> MMVAWWSLFLYGLQVAAPALAATPADWRSQSIYFLLTDRFARTDGSTTATCNTADQKYCGG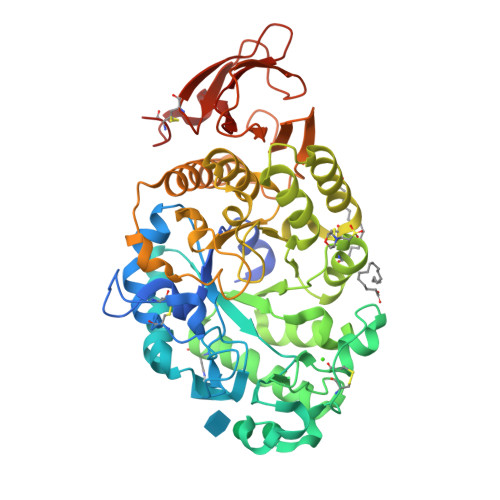TWQGIIDKLDYIQGMGFTAIWITPVTAQLPQTTAYGDAYHGYWQQDIYSLNENYGTADDLKALSSALHERGMYLMVDVVANHMGYDGAGSSVDYSVFKPFSSQDYFHPFCLIQNYEDQTQVEDCWLGDNTVSLPDLDTTKDVVKNEWYDWVGSLVSNYSIDGLRIDTVKHVQKDFWPGYNKAAGVYCIGEVLDGDPAYTCPYQNVMDGVLNYPIYYPLLNAFKSTSGSMDDLYNMINTVKSDCPDSTLLGTFVENHDNPRFASYTNDIALAKNVAAFIILNDGIPIIYAGQEQHYAGGNDPANREATWLSGYPTDSELYKLIASANAIRNYAISKDTGFVTYKNWPIYKDDTTIAMRKGTDGSQIVTILSNKGASGDSYTLSLSGAGYTAGQQLTEVIGCTTVTVGSDGNVPVPMAGGLPRVLYPTEKLAGSKICSSS N,N-dimethyl-L-histidine | C8 H13 N3 O2 | 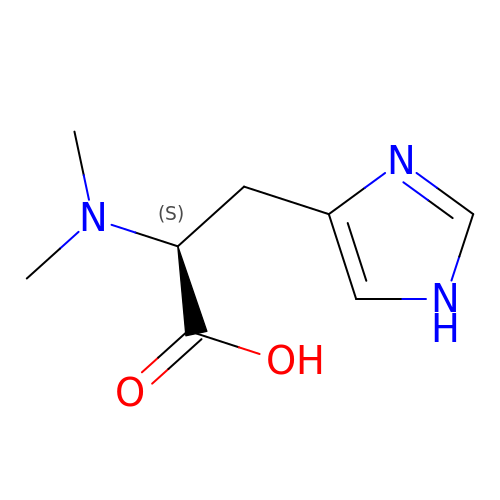IMOBSLOLPCWZKQ-ZETCQYMHSA-N>[2x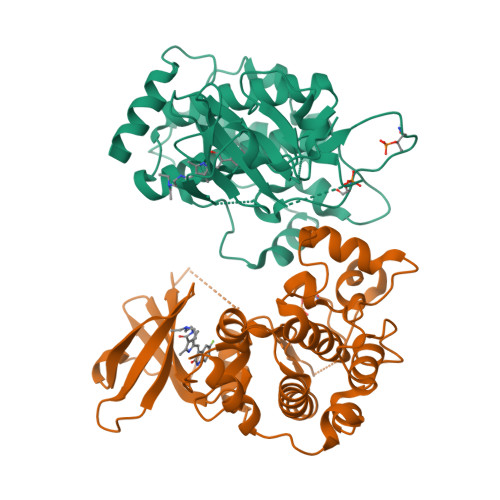]GSMDVVDPDIFNRDPRDHYDLLQRLGGGTYGEVFKARDKVSGDLVALKMVKMEPDDDVSTLQKEILILKTCRHANIVAYHGSYLWLQKLWICMEFCGAGSLQDIYQVTGSLSELQISYVCREVLQGLAYLHSQKKIHRDIKGANILINDAGEVRLADFGISAQIGATLARRLSFIGTPYWMAPEVAAVALKGGYNELCDIWSLGITAIELAELQPPLFDVHPLRVLFLMTKSGYQPPRLKEKGKWSAAFHNFIKVTLTKSPKKRPSATKMLSHQLVSQPGLNRGLILDLLDKLKNPGKGPSIGDIEDEE>[6x]MRLELPVIPLRNTVILPHTTTPVDVGRAKSKRAVEEAMGADRLIFLVAQRDPEVDDPAPDDL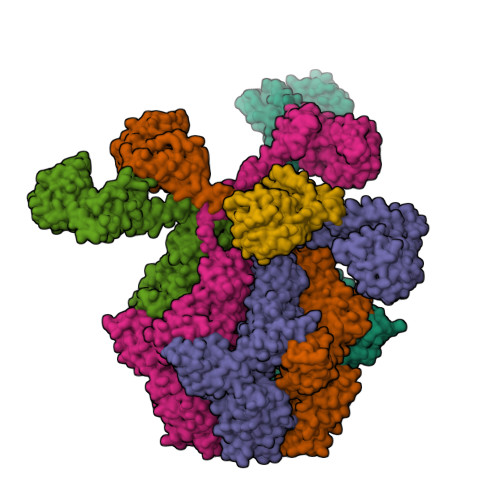YTWGVQAVVKQAMRLPDGTLQVMVEARARAQVTDYIPGPYLRARGEVFSEIFPIDEAVVRVLVEELKEAFEKYVANHKSLRLDRYQLEAVKGTSDPAMLADTIAYHATWTVAEKQEILELTDLEARLKKVLGLLSRDLERFELDKRVAQRVKEQMDTNQREYYLREQMKAIQKELGGEDGLSDLEALRKKIEEVGMPEAVKTKALKELDRLERMQQGSPEATVARTYLDWLTEVPWSKADPEVLDINHTRQVLDEDHYGLKDVKERILEYLAVRQLTQGLDVRNKAPILVLVGPPGVGKTSLGRSIARSMNRKFHRISLGGVRDEAEIRGHRRTYIGAMPGKLIHAMKQVGVINPVILLDEIDKMSSDWRGDPASAMLEVLDPEQNNTFTDHYLDVPYDLSKVFFITTANTLQTIPRPLLDRMEVIEIPGYTNMEKQAIARQYLWPKQVRESGMEGRIEVTDAAILRVISEYTREAGVRGLERELGKIARKGAKFWLEGAWEGLRTIDASDIPTYLGIPRYRPDKAETEPQVGTAQGLAWTPVGGTLLTIEVAAVPGSGKLSLTGQLGEVMKESAQAALTYLRAHTQDYGLPEDFYNKVDLHVHVPDGATPKDGPSAGITMATAIASALSRRPARMDIAMTGEVSLRGKVMPIGGVKEKLLAAHQAGIHKIVLPKDNEAQLEELPKEVLEGLEIKLVEDVGEVLEYLLLPEPTMPPVVQPSDNRQQPGAGAKLAAALEHHHHHH Bacteriophage E217 infects Pseudomonas aeruginosa and is part of an experimental phage cocktail developed to eradicate P. aeruginosa infections in Galleria mellonella (wax moth) larvae and vertebrate models. E217 is a PB1-like Myoviridae of the Pbunavirus genus characterized by a ~66.2 kbp genome, significantly smaller than the classical enterobacteria phage T4 (~169 kbp). Here, we describe the structure of the whole E217 virion before and after DNA ejection at 3.1 Å and 4.5 Å resolution, respectively, determined using cryogenic electron microscopy (cryo-EM). We identify and build de novo structures for 19 unique E217 gene products, resolve the tail genome-ejection machine in both extended and contracted states, and decipher the complete architecture of the baseplate formed by 66 polypeptide chains.

We reconstructed the E217 head using alocalized reconstruction with fivefold symmetry imposed (C5), which yielded 2.8 Å resolution at 0.143 cut-off Fourier Shell Correlation (FSC). The E217 head has a maximum diameter of 790 Å and is built by 535 copies of the major capsid protein gp25. We will refer to the reconstruction of the E217 virion at neutral pH with an extended tail that was determined at an FSC = 0.143 resolution of 2.8 Å, although no significant differences were observed in the E217 head because of alkalization. The first 65 amino acids of gp25 were not visible in the reconstruction, suggesting this moiety could be cleaved during maturation or is disordered in our reconstruction. We found that E217 has a T = 9 icosahedral capsid decorated by gp24, a likely cementing protein stabilizing the E217 capsid. Each gp24 subunit consists of two anti-parallel β-sheets, arranged like the petals of a flower, to form a tulip-like structure. Each E217 gp24 trimer contacts three neighboring decorating proteins and six capsid protein subunits in three adjacent capsomers, burying a total surface area of ~8642 Å2. Gp24 trimers at neighboring threefold/quasi-threefold axes generate an inter-capsomer cage. The interconnected architecture of gp24 trimers is stabilized by extensive van der Waals contacts between N-terminal arms and omega loops.

>[11x]NFTAPVTTPSIPTPIQFLQTWLPGFVKVMTAARKIDEIIGIDTVGSWEDQEIVQGIVEPAGTAVEYGDHTNIPLTSWNANFERRTIVRGELGMMVGTLEEGRASAIRLNSAETKRQQAAIGLETFRNAIGFYGWQSGLGNRTYGFLNDPNLPAFQTPPSQGWSTADWAGIIGDIREAVRQLRIQSQDQIDPKAEKITLALATSKVDYLSVTTPYGISVSDWIEQTYPKMRIVSAPELSGVQMKNQEPEDALVLFVEDVNAAVDGSTDGGSVFSQLVQSKFITLGVEKRAKSYVEDFSNGTAGALCKRPWAVVRYLGI;>MFQKQVYRQYTPGFPGDLIEDGPKRARPGRIMSLSAVNPAATATGPNRASRAFGYAGDVSALGEGQPKTIAARASEVVIGGANFFGVLGHPKHYALFGSAGDSLAPSYDLPDGAEGEFFDMATGLVVEIFNGAAAALDLDYGDLVAYVPNNLATADDALGLPAGALVGFKTGSMPTGLVQIPNARIVNAISLPAQSAGNLVAGVTIVQLTQ[3x]4-{8-amino-3-[(6R,8aS)-3-oxohexahydro-3H-[1,3]oxazolo[3,4-a]pyridin-6-yl]imidazo[1,5-a]pyrazin-1-yl}-N-[4-(trifluoromethyl)pyridin-2-yl]benzamide 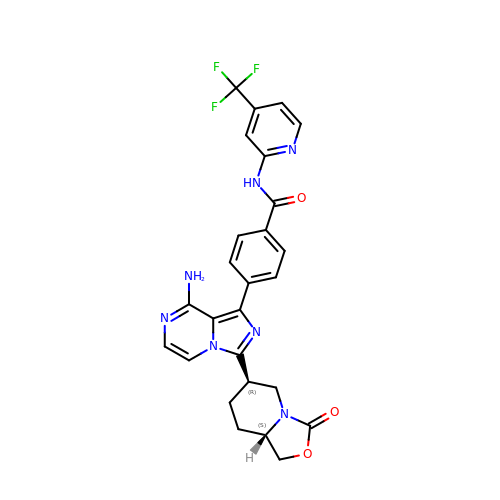| C26 H22 F3 N7 O3 | CDISOBGWDHAHGF-AEFFLSMTSA-N> GSWEIDPKDLTFLKELGTGQFGVVKYGKWRGQYDVAIKMIKEG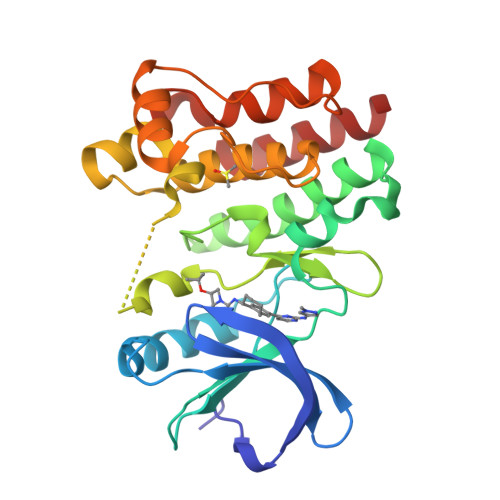SMSEDEFIEEAKVMMNLSHEKLVQLYGVCTKQRPIFIITEYMANGCLLNYLREMRHRFQTQQLLEMCKDVCEAMEYLESKQFLHRDLAARNCLVNDQGVVKVSDFGLSRYVLDDEYTSSVGSKFPVRWSPPEVLMYSKFSSKSDIWAFGVLMWEIYSLGKMPYERFTNSETAEHIAQGLRLYRPHLASEKVYTIMYSCWHEKADERPTFKILLSNILDVMDEES>MMDKFRMIFQFLQSNQESFMNGICGIMALASAQMYSAFDFNCPCLPGYNAAYSAGILLAPPLVLFLLGLVMNNNVSMLAEEWKRPPGRRAKDPAVLRYMFCSMAQRALWAPVVWVAVTLLDGKCFLCAFCTAVPVSALGNGSLAPGLPAPELARLLARVPCPEIYDGDWLLAREVAVRYLRCISQALGWSFVLLTTLLAFVVRSVRPCFTQAAFLKSKYWSHYIDIERKLFDETCTEHAKAFAKVCIQQFFEAMNHDLELGHTNGTLATAPASAAAPTTPDGAEEEREKLRGITDQGTMNRLLGSAWSHPQFEK[8x]

Calcium homeostasis modulator 1 (CALHM1) is a voltage-dependent channel involved in neuromodulation and gustatory signaling. CALHM1 is the recently identified member of a large-pore channel that permeates ions, including Ca2+, Na+, K+, and Cl−, and small molecules, such as ATP, in a voltage-dependent manner. Furthermore, the ATP efflux through the CALHM1 channel in type II gustatory cells and the subsequent purinergic signaling has been shown to facilitate the perception of sweet, bitter, and umami taste sensations. Our studies here showed that the human and chicken CALHM1s have a conserved structural fold, oligomeric assembly pattern, and a phospholipid-filled hydrophobic pocket for controlling channel functions.

The single-particle cryo-EM on hCALHM1I109W∆ct in the presence of RuR showed oblong density consistent with the size of RuR in the central pore surrounded by the NTHs. The resolution of the cryo-EM map is lower around the NTHs and pore region compared to the TMDs, possibly suggesting a number of subtly different binding modes within this binding pocket since the pore diameter is large. Nevertheless, the cryo-EM density is of sufficient quality for the placement of RuR molecule, although an atomic-resolution pose cannot be determined from these data. The RuR molecule is positioned to plug the pore through associations with the NTHs. To validate this structural observation, we mutated the pore-lining residues proximal to RuR to arginine (Gln10Arg, Gln13Arg, and Gln16Arg) and assessed RuR-mediated channel blockade by patch-clamp electrophysiology. We reasoned that arginine residues that face the pore of the channel, being positively charged and bulkier than glutamine, would disfavor binding of the positively charged RuR and decrease the extent of channel blockade. Indeed, the Gln10Arg, Gln13Arg, and Gln16Arg mutants all decreased the extent of channel blockade to different extents. Thus, the experiments above validated our structural observation that RuR binds and plugs the central pore formed by the NTHs. Our hCALHM1 structure shows that NTHs are positioned approximately orthogonal to the membrane plane and that RuR binds to the pore generated by the NTHs from the eight subunits.>[2x]GPGSDAEQRAVAKALFDAVNKHLSNPFIEVEMRLGQFKVEEDANFTACVSTEDYERIKTYLMTEMENSSMTRSVTHDVSL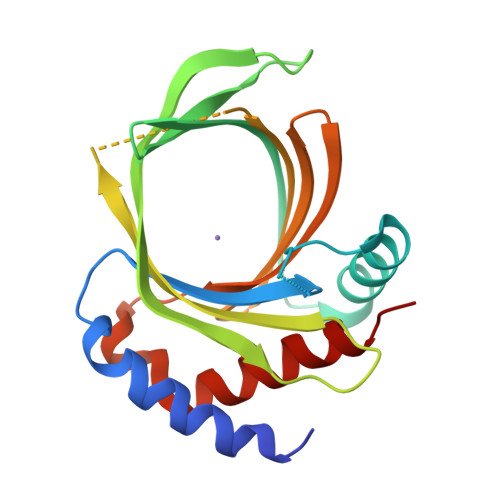RGWRHTYATDENGNPTRCVSIVRKKRLFVKNIVVPLGAYNLRFAVSTETPGDLRFSGAGPRAGHTRLKDRLSITDGMFRYDMTQVTEKGVLMHEVEIEGVFSSHEKQLTESWLEELLRRAMRLATLRTN>SNAESAAPQVHLSILATTDIHANMMDYDYYSDKETADFGLARTAQLIQKHREQNPNTLLVDNGDLIQGNPLGEYAVKYQKDDIISGTKTHPIISVMNALKYDAGTLGNHEFNYGLDFLDGTIKGADFPIVNANVKTTSGENRYTPYVINEKTLIDENGNEQKVKVGYIGFVPPQIMTWDKKNLEGQVQVQDIVESANETIPKMKAEGADVIIALAHTGIEKQAQSSGAEN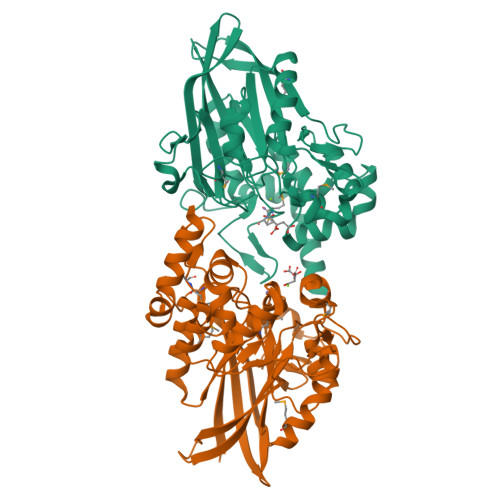AVFDLATKTKGIDAIISGHQHGLFPSAEYAGVAQFNVEKGTINGIPVVMPSSWGKYLGVIDLKLEKADGSWKVADSKGSIESIAGNVTSRNETVTNTIQQTHQNTLEYVRK[2x]> QSISPNELGLTSAQDDGPLGNEKPNYFLNFRTMNVDIFTVSHTKVDNIFGRAWYVASHDFNNGDTWRQKLTFPKEGHGMLSQFFAYFTGEINIHILYMAEQGFLRVAHTYDTEDNRKTFLSSNGVITIPAGEQMTLSVPFYSNKPLRTVRHDSALGFLMCRPMMHGTTRTTAEVYISLRCPNFFFPVPAPKPTGSRAA;> TKYKWTRTKVDIAEGPGTMNMANVLSTTGAQSVALVGERAFYDPRTAGSKSRFDDMIKIAQLFSVMSDNTTPSSSSGIDKYGYFDWAATVAPQNMVHRNVVTLDQFPNLNLFMNTYSYFRGSLIIRLSIYASTFNRGRLRMGFFPNCTHDTQLELDNAIYTICDIGSDNSFELTIPYSFSTWMRKTHGHQLGLFQVEVLNRLTYNSSSPNKVHCIVQGRLGDDAKFFCPTGSLVSFQ;> LSNVETEANNIISGNEVGGEIITKVADDASNLLGPNSFATTAQPENKDVVQATTTVNTTNLTQHPSAPTIPFTPDFRNVDNFHSMAYDITTGDKNPSKLIRLDTASWQTSYSRQYKITTVELPKSFWDDTRKPAYGQAKYFAAVRCGFHFQVQVNVNQGTAGSALVVYEPKPVIDSRQYLEFGSLTNLPHVLMNLAETTQADLCIPYVADTNYVKTDSSDLGQLRVYVWTPLSVPTGASNEVDVTVMGSLLQLDFQNPRPYGE

However, an emerging pathogen, human parechovirus 3 (HPeV3) can cause severe central nervous system infections such as meningitis, and is a leading cause of neonatal sepsis. We utilized cryo-electron microscopy and image reconstruction to analyse the structure of HPeV3 on its own and in complex with a human monoclonal antibody Fab. The HPeV3 capsid is composed of 60 copies of three β-jellyroll proteins, VP0, VP1 and VP3 in a T=1, pseudo T=3 arrangement. The virion structure shows that VP1 pocket-binding drugs, such as pleconaril, are unlikely to bind to HPeV; that VP0 is an important protein for stabilizing the inner surface of the capsid, and finally, that the assembly of HPeV is most likely controlled by multiple interactions of the genome with the capsid, through conserved amino acids in VP1 and VP3 and stem-loop structures in the RNA.

We determined a 4.3 Å resolution HPeV3 structure using electron cryo-microscopy and single particle analysis. Homology models of capsid proteins VP0, VP1 and VP3 were used as starting models to generate an atomic model of HPeV3 constrained by the density from the reconstruction. Unusually for a picornavirus, we showed by polyacrylamide gel electrophoresis protein analysis and from the structure, that VP0 does not undergo autocatalytic cleavage into VP4 (N-terminal) and VP2 (C-terminal) in the virion. Similar to many picornaviruses, HPeV3 possesses an open channel at each fivefold vertex and a canyon for potential receptor and antibody binding, however, it is wide and shallow. Five VP3 N termini come together to form an annulus at the base of the channel, giving intra-pentamer stability. Instead the VP0 N terminus straddles an adjacent threefold on the inner surface of the capsid, forming a loop that stabilises the twofold-related VP0 from another pentamer (pentamers 1 and 3), a conformation that has not been previously observed to our knowledge. Unusually, about 25% of the genomic RNA is highly ordered, and at high occupancy in the reconstruction. Finger-like RNA densities come into close contact with capsid proteins VP1 and VP3 around the vertices that could accommodate about 30 nucleotides. Moreover, we identified the conserved regions in the N terminus of VP3 (T20-R26, T47-T65), hZ helix and the βIC terminus regions of VP1 (R202-N205) as the structured RNA interaction sites. We revealed the unusual stability of these capsids at the intra-pentamer level by VP3 interactions and at the inter-pentamer by VP0, and propose that the uncoating mechanism of the HPeV genome will be significantly different to that of other picornaviruses.>[4x]MPLLLLLPLLWAGALAELHHHHHHENLYFQSGRYKCGISKACPEK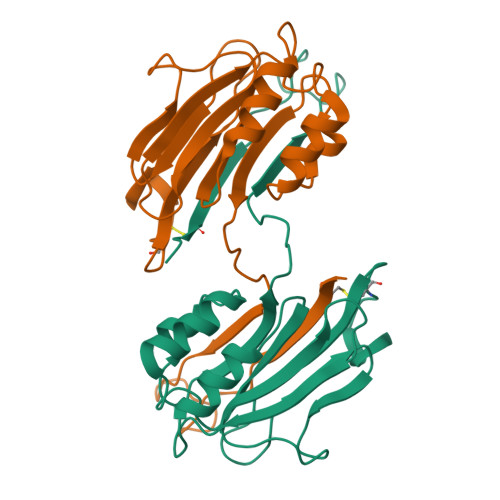HFAFKMASGAANVVGPKICLEDNVLMSGVKNNVGRGINIALVNGKTGEVIDTKFFDMWGGDVAPFIEFLKTIQDGTVVLMATYDDGATKLTDEARRLIAELGSTSITSLGFRDNWVFCGGKGIKTKSPFEQHIKNNKETNKYEGWPEVVEMEGCIPQKQD> SEDCENIFHDNAYLLKLDCEAGRVDPVEFDDISDEEIYEITVDVGVSSED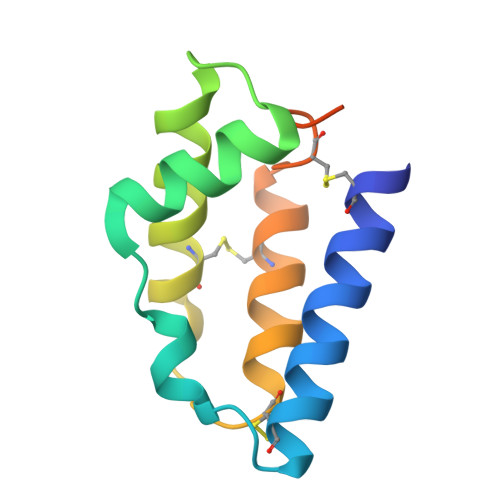QEKVAKIIRECIAQVSTQDCTKFSEIYDCYMKKKICNYYPENMGSGHHHHHHHH2-({2-[(4-carboxyphenyl)amino]pyrimidin-4-yl}amino)benzoic acid | C18 H14 N4 O4 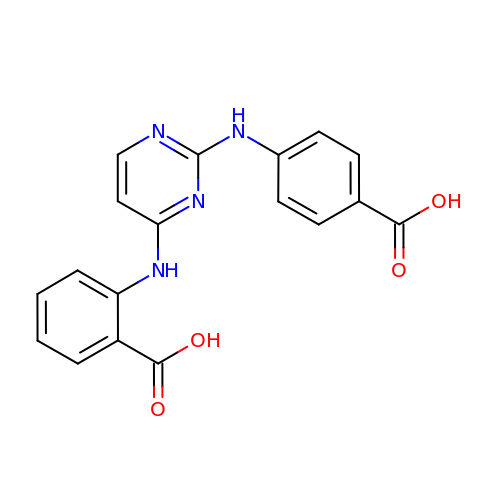| UIAQHDUGAOFVJM-UHFFFAOYSA-N> MRRLEEDAVRVAYAGLRRKEAFKALAEKLGFTPLLFPVQATEKVPVPEYRDQVRALAQGVDLFLATTGVGVRDLLEAGKALGLDLEGPLAKAFRLARGAKAARALKEAGLPPHAVGDGTSKSLLPLLPQGRGVAALQLYGKPLPLLENALAERGYRVLPLMPYRHLPDPEGILRLEEA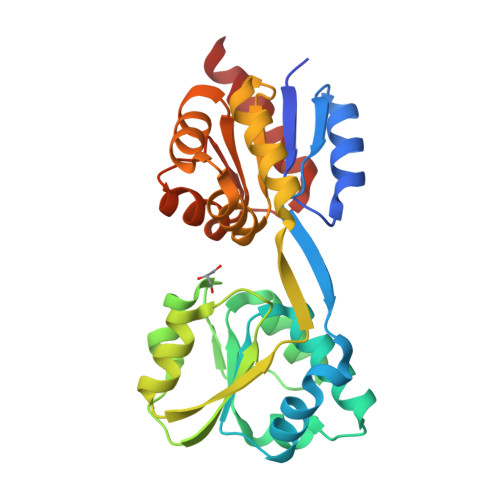LLRGEVDALAFVAAIQVEFLFEGAKDPKALREALNTRVKALAVGRVTADALREWGVKPFYVDETERLGSLLQGFKRALQKEVA>GAMVSQPIKLLVGLANPGPEYAKTRNNAGAWVVEELARIHNVTLKNEPKFFGLTGRLLINSQELRVLIPTTFMNLSGKAIAALANFYQIKPEEIMVAHDELDLPPGVAKFKQGGGHGGHNGLKDTISKLG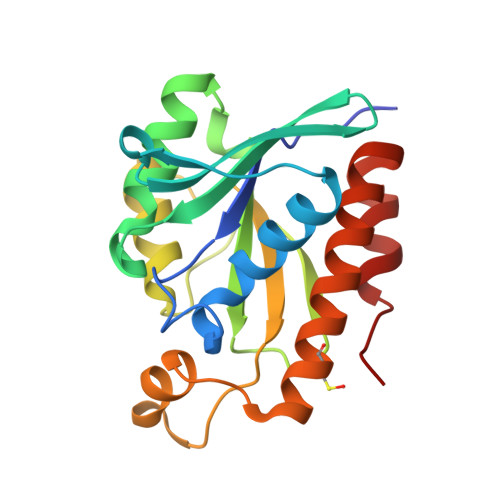NNKEFYRLRLGIGHPGHKDKVAGYVLGKAPAKEQECLDAAVDESVRCLEILMKDGLTKAQNRLHTFKAE[2x]>[2x]MNILAIDIGGTMIKYGLVSFDGKILSTDKIKTEASKGLNNILNKIDNIFKRYKENNPVGIAVSGTGQINGMIGKVIGGNPIIPNWIGTNLVKILEEKYNLPIVLENDVNCVALGEKWVGAGKDLSNFICLTIGTGIGGGILLNNQLFRGEN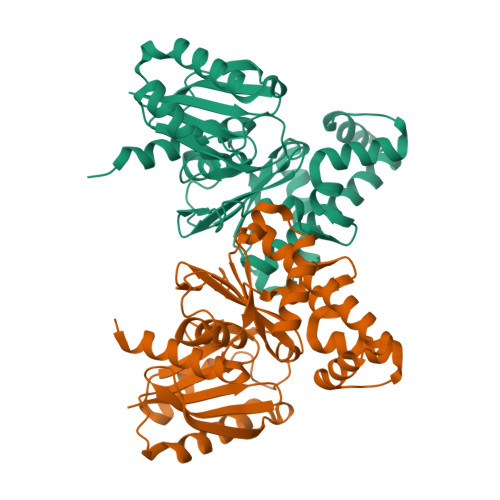FVAGEFGHILIKKGEFEQFASTTALIRLVKERTGKTLNGKEIFDLEKKEILEYQEIISEWIENLTDGLSSIIYCFNPANIILGGGVIEQGEPLINRIKNSLFKKIGPQFKEKLNITQAKLGNNAGMIGASYLLLEKINKR>[4x]MRGGALL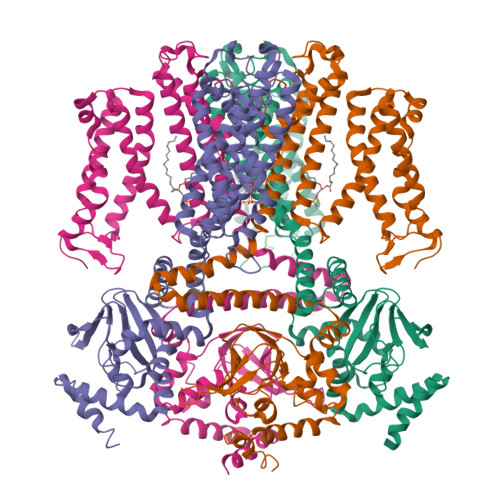CGQVQDEIEQLSRESSHFSLSTGILPSLGARSNRRVKLRRFVVSPYDHKYRIWEAFLVVLVVYTAWVSPFEFGFLRKPRPPLSITDNIVNAFFAIDIIMTFFVGYLDKSTYLIVDDRKQIAFKYLRSWFLLDLVSTIPSEAAMRISSQSYGLFNMLRLWRLRRVGALFARLEKDRNFNYFWVRCAKLVCVTLFAVHCAACFYYLIAARNSNPAKTWIGANVANFLEESLWMRYVTSMYWSITTLTTVGYGDLHPVNTKEMIFDIFYMLFNLGLTAYLIGNMTNLVVHGTSRTRNFRDTIQAASNFAHRNHLPPRLQDQMLAHLCLKYRTDSEGLQQQETLDALPKAIRSSISHFLFYSLMDKVYLFRGVSNDLLFQLVSEMKAEYFPPKEDVILQNEAPTDFYILVNGTADLVDVDTGTESIVREVKAGDIIGEIGVLCYRPQLFTVRTKRLCQLLRMNRTTFLNIIQANVGDGTIIMNNLLQHLKEMNDPVMTNVLLEIENMLARGKMDLPLNLCFAAIREDDLLLHQLLKRGLDPNESDNNGRTPLHIAASKGTLNCVLLLLEYHADPNCRDAEGSVPLWEAMVEGHEKVVKVLLEHGSTIDAGDVGHFACTAAEQGNLKLLKEIVLHGGDVTRPRATGTSALHTAVCEENIEMVKYLLEQGADVNKQDMHGWTPRDLAEQQGHEDIKALFREKLHERRVHIETSSSVPILKTGIRFLGRFTSEPNIRPASREVSFRIRETRARRKTNNFDNSLFGILANQSVPKNGLATVDEGRTGNPVRVTISCAEKDDIAGKLVLLPGSFKELLELGSNKFGIVATKVMNKDNNAEIDDVDVIRDGDHLIFATDSLEGSDEVDAGSAAASGGSDYKDDDDKGSHHHHHHHHHH> GSGSWEIDPKDLTFLKELGTGQFGVVKYGKWRGQYDVAIKMIKEGSMSEDEFIEEAKVMMNLSHEKLVQLYGVCTKQRPIFIITEYMANGCLLNYLREMRHRFQTQQLLEMCKDVCEAMEYLESKQFLHRDLAARNCLVNDQGVVKVSDFGLSRYVLDDEYTSSVGSKFPVRWS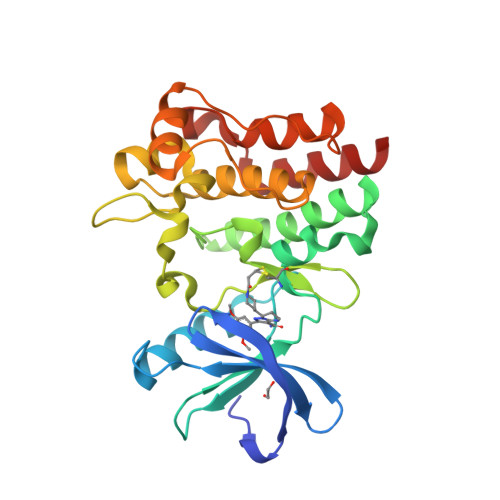PPEVLMYSKFSSKSDIWAFGVLMWEIYSLGKMPYERFTNSETAEHIAQGLRLYRPHLASEKVYTIMYSCWHEKADERPTFKILLSNILDVMDEES> PNITLKIIETYLGRVPSVNEYHMLKSQARNIQKITVFNKDIFVSLVKKNKKRFFSDVNTSASEIKDRILSYFSKQTQTYNIGKLFTIIELQSVLVTTYTDILGVLTIKAPNVISSKISYNVTSMEELARDMLNSMNVAVIDKAKVMGRHNVSSLVKNVNKLMEEYLRRHNKSCICYGSYSLYLINPNIRYGDIDILQTNSRTFLIDLAFLIKFITG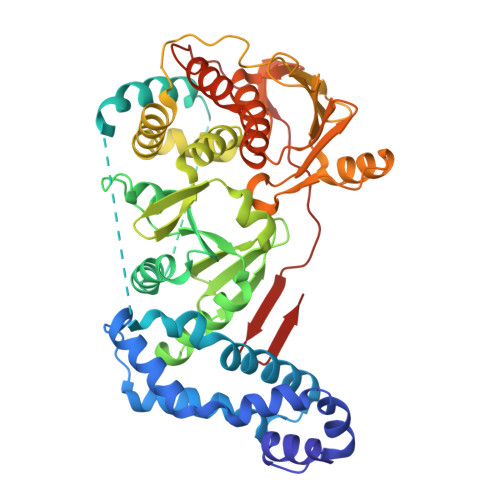NNIILSKIPYLRNYMVIKDENDNHIIDSFNIRQDTMNVVPKIFIDNIYIVDPTFQLLNMIKMFSQIDRLEDLSKDPEKFNARMATMLEYVRYTHGIVFDGKRNNMPMKCIIDENNRIVTVTTKDYFSFKKCLVYLDENVLSSDILDLNADTSCDFESVTNSVYLIHDNIMYTYFSNTILLSDKGKVHEISARGLCAHILLYQMLTSGEYKQCLSDLLNSMMNRDKIPIYSHTERDKKPGRHGFINIEKDIIVF> MKILLIGMGGTIASVKGENGYEASLSVKEVLDIAGIKDCEDCDFLDLKNVDSTLIQPEDWVDLAETLYKNVKKYDGIIVTH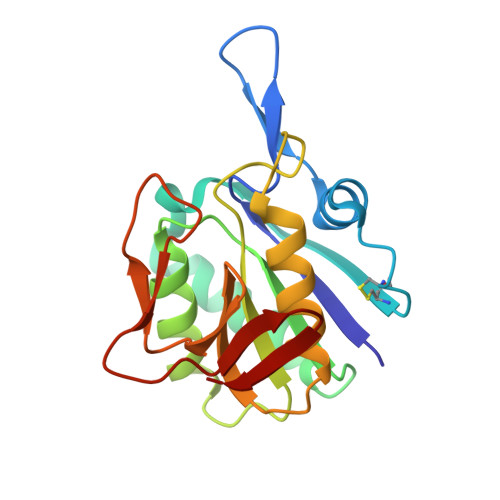GTDTLAYTSSMISFMLRNPPIPIVFTGSMIPATEENSDAPLNLQTAIKFATSGIRGVYVAFNGKVMLGVRTSKVRTMSRDAFESINYPIIAELRGEDLVVN>GAMAGVFTYETEFTSVIPPPRLFKAFILDADNLIPKIAPQAVKCAEIIAGAGGVGTIKKITFGEGSQFGSVTHKIDGIDKENFVYSYSLIEGDALSDKIEKISYETKLVSSSDGGSIIKSTSNYHTKGDVEIKEE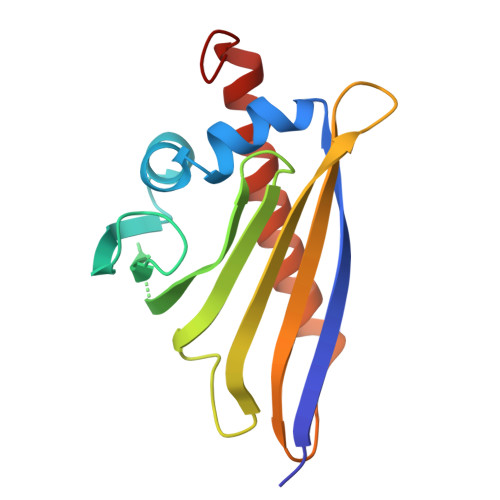HVKAGKEKASHLFKLVEGYLLANPNEYC[2x]> MPTYIELINIVNDDTPEDDAVISDLMSQMNDKQTVLDSCRINHKGNAYFKFHVK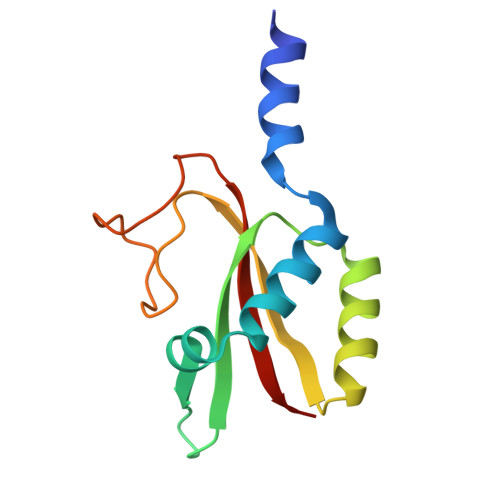GSISKDKLKALNETLKDSNLVVTDASTQRGFMPPNKFDDITYTEESVGYRAMVWTSFTIEKLLV>[2x]MHHHHHHLPNITILATGGTIAGGGDSATKSNYTVGKVGVENLVNAVPQLKDIANVKGEQVVNIGSQDMNDNVWLTLAKKINTDCDKTDGFVITHGTDTMEETAYFLDLTVKCDKPVVMVGAMRPSTSMSADGPFNLYNAVVTAADKASANRGVLVVMNDTVLDGRDVTMTNTTDVATFKSVNYGPLGYIHNGKIDYQRTPARKHTSDTPFDVSKLNELPKVGIVYNYANASDLPAKA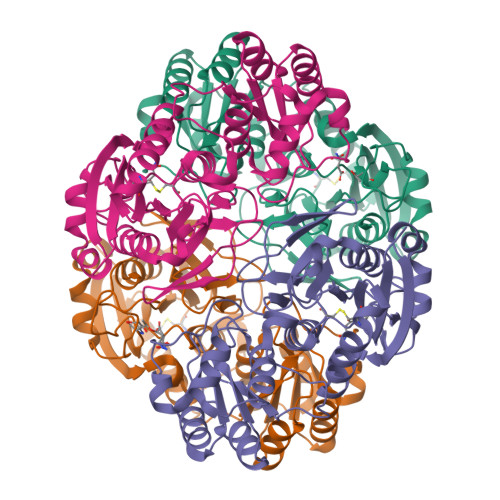LVDAGYDGIVSAGVGNGNLYKSVFDTLATAAKTGTAVVRSSRVPTGATTQDAEVDDAKYGFVASGTLNPQKARVLLQLALTQTKDPQQIQQIFNQY;>MHHHHHHLPNITILATGGDIAGGGDSATKSNYTVGKVGVENLVNAVPQLKDIANVKGEQVVNIGSQDMNDNVWLTLAKKINTDCDKTDGFVITHGTDTMEETAYFLDLTVKCDKPVVMVGAMRPSTSMSADGPFNLYNAVVTAADKASANRGVLVVMNDTVLDGRDVTMTNTTDVATFKSVNYGPLGYIHNGKIDYQRTPARKHTSDTPFDVSKLNELPKVGIVYNYANASDLPAKALVDAGYDGIVSAGVGNGNLYKSVFDTLATAAKTGTAVVRSSRVPTGATTQDAEVDDAKYGFVASGTLNPQKARVLLQLALTQTKDPQQIQQIFNQY[2x]>MAKHLFTSESVSEGHPDKIADQISDAVLDAILEQDPKARVACETYVKTGMVLVGGEITTSAWVDIEEITRNTVREIGYVHSDMGFDANSCAVLSAIGKQSPDINQGVDRADPLEQGAGDQGLMFGYATNETDVLMPAPITYAHRLVQRQAEVRKNGTLPWLRPDAKSQVTFQYDDGKIVGIDAVVLSTQHSEEIDQKSLQEAVMEEIIKPILPAEWLTSATKFFINPTGRFVIGGPMGDCGLTGRKIIVDTYGGMARHGGGAFSGKDPSKVDR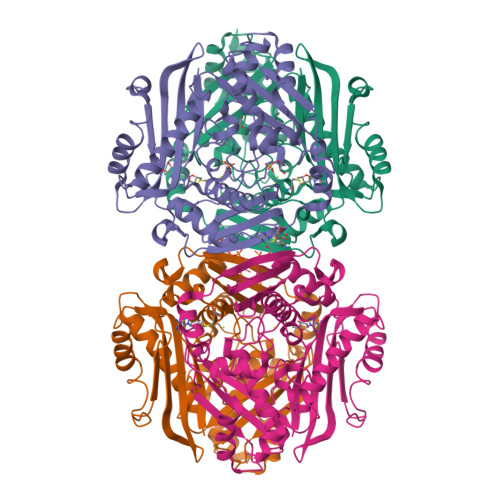SAAYAARYVAKNIVAAGLADRCEIQVSYAIGVAEPTSIMVETFGTEKVPSEQLTLLVREFFDLRPYGLIQMLDLLHPIYKETAAYGHFGREHFPWEKTDKAQLLRDAAGLK[4x]>[3x]M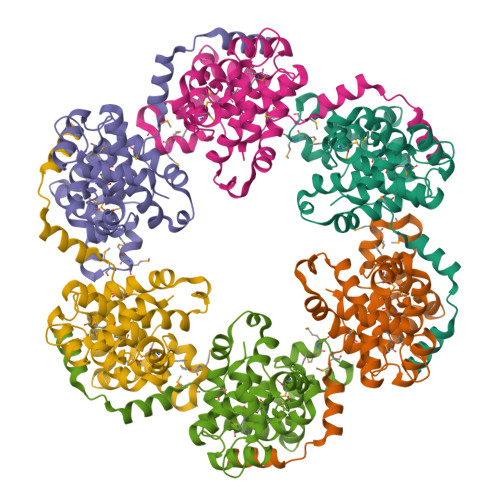DNYQELRVQFAAQAVDRNEIEQWVREFAYQGFDARRVIELLKQYGGADWEKDAKKMIVLALTRGNKPRRMMMKMSKEGKATVEALINKYKLKEGNPSRDELTLSRVAAALAGWTCQALVVLSEWLPVTGTTMDGLSPAYPRHMMHPSFAGMVDPSLPGDYLRAILDAHSLYLLQFSRVINPNLRGRTKEEVAATFTQPMNAAVNSNFISHEKRREFLKAFGLVDSNGKPSAAVMAAAQAYKTAA>[2x]DYKDDDDKLAAAQYPVVNTNYGKIRGLRTPLPNEILGPVEQYLGVPYASPPTGERRFQPPEPPSSWTGIRNTTQFAAVCPQHLDERSLLHDMLPIWFTANLDTLMTYVQDQNEDCLYLNIYVPTEDDIHDQNSKKPVMVYIHGGSYMEGTGNMIDGSILASYGNVIVI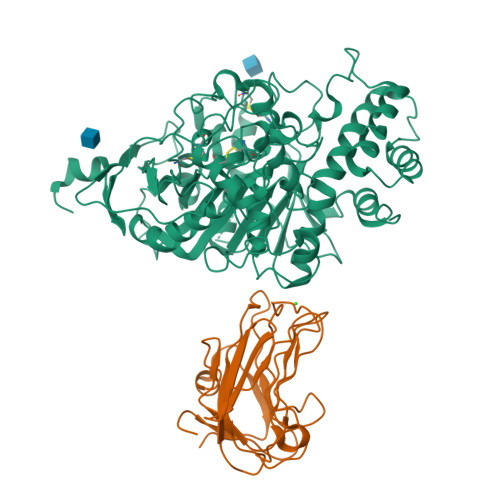TINYRLGILGFLSTGDQAAKGNYGLLDQIQALRWIEENVGAFGGDPKRVTIFGSGAGASCVSLLTLSHYSEGLFQKAIIQSGTALSSWAVNYQPAKYTRILADKVGCNMLDTTDMVECLRNKNYKELIQQTITPATYHIAFGPVIDGDVIPDDPQILMEQGEFLNYDIMLGVNQGEGLKFVDGIVDNEDGVTPNDFDFSVSNFVDNLYGYPEGKDTLRETIKFMYTDWADKENPETRRKTLVALFTDHQWVAPAVATADLHAQYGSPTYFYAFYHHCQSEMKPSWADSAHGDEVPYVFGIPMIGPTELFSCNFSKNDVMLSAVVMTYWTNFAKTGDPNQPVPQDTKFIHTKPNRFEEVAWSRYNPKDQLYLHIGLKPRVRDHYRATKVAFWLELVPHLHNLNEIFQYVSTTTKVPPPDMT;>[2x]GGHAGTTYIFSKGGGQITYKWPPNDRPSTRADRLAIGFSTVQKEAVLVRVDSSSGLGDYLELHIHQGKIGVKFNVGTDDIAIEESNAIINDGKYHVVRFTRSGGNATLQVDSWPVIERYPAGRQLTIFNSQATIIIGGKEQGQPFQGQLSGLYYNGLKVLNMAAENDANIAIVGNVRLV> MHKLIIKYNKQLKMLNLRDGKTYTISEDERADITLKSLGEVIHLEQNNQGTWQANHTSINKVLVRKGDL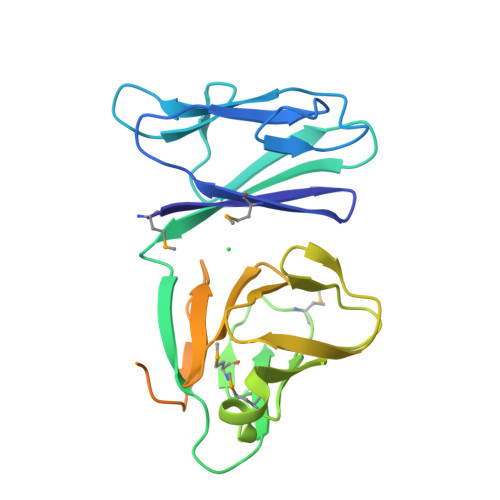DDITLQLYTEADYASFAYPSIQDTMTIGPNAYDDMVIQSLMNAIIIKDFQSIQESQYVRIVHDKNTDVYINYELQEQLTNKAYIGDHIYVEGIWLEVQADGLNVLSQNTVASSLIRLTQEMPHAQADDYNTYHRSPRIIHREPTDDIKIERPPQPIQKNNTLEHHHHHH> PVCVRPTPK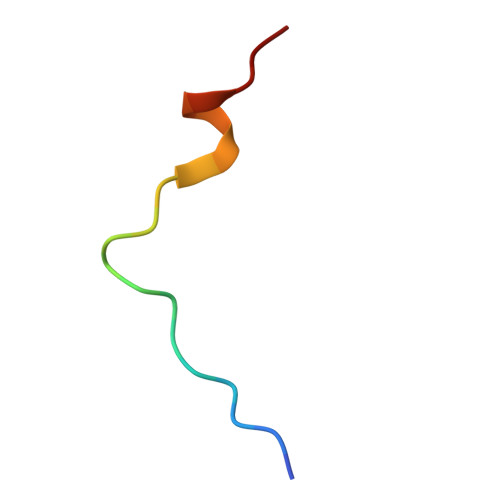WQKGIGEFFRL>ATAAEIAALPRQKVELVDPPFVHAHSQVAEGGPKVVEFTMVIEEKKIVIDDAGTEVHALAFNGTVPGPLMVVHQDDYLELTLINPETNTLMHNIDFHAATGALGGGGLTEINPGEKTILRFKATKPGVFVYHCAPPGMVPWHVVSGMNGAIMVLPREGLHDGKGKALTYDKIYYVGEQDFYVPRDENGKYKKYEAPGDAYEDTVKVMRTLTPTHVVFNGAVGALTGDKAMTAAVGEKVLIVHSQANRDTRPHLIGGHGDYVWATGKFNTPPDVDQETWFIPGGAAGAAFYTF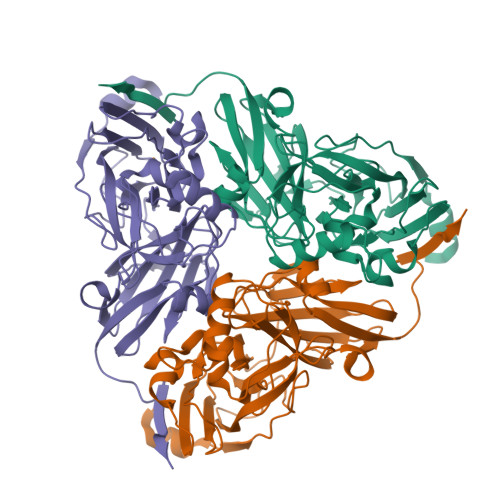QQPGIYAYVNHNLIEAFELGAAAHFKVTGEWNDDLMTSVLAPSG[3x]> TITGDTCNEETQNLSTIYLREYQSKVKRQI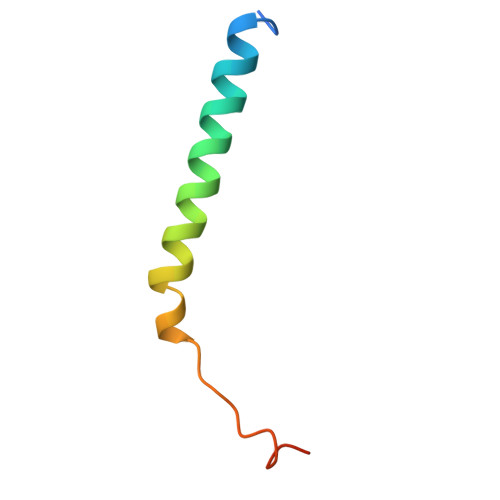FSDYQSEVDIYNRIRDEL> GGFVAHVESTCLLDDAGTPKDFTYCISFNKDLLTCWDPEENKMAPCEFGVLNSLANVLSQHLNQKDTLMQRLRNGLQNCATHTQPFWGSLTNRTRPPSVQVAKTTPFNTREPVMLACYVWGFYPAEVTITWRKNGKLVMPHSSAHKTAQPNGDWTYQTLSHLALTPSYGDTYTCVVEHIGAPEPILRD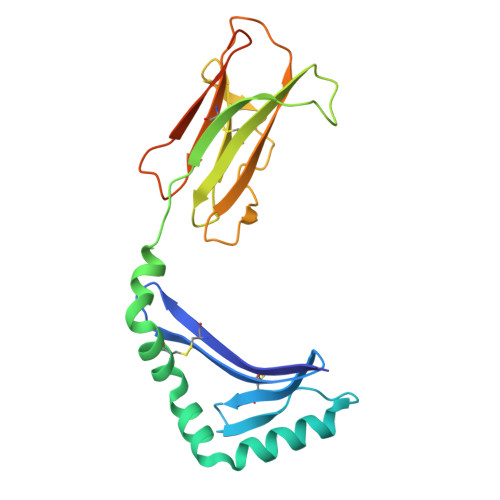WTPGLSPMQTLKKPPTPPPEPET>[4x]MSQHNEKNPHQHQSPLHDSSEAKPGMDSLAPEDGSHRPAAEPTPPGAQPTAPGSLKAPDTRNEKLNSLEDVRKGSENYALTTNQGVRIADDQNSLRAGSRGPTLLEDFILREKITHFDHERIPERIVNARGSAAHGYFQPYKSLSDITKADFLSDPNKITPVFVRFSTVQGGAGSADTVRDIRGFATKFYTEEGIFDLVGNNTPIFFIQDAHKFPDFVHAVKPEPHWAIPQGQSAHDTFWDYVSLQPETLHNVMWAMSDRGIPRSYRTMEGFGIHTFRLINAEGKATFVRFHWKPLAGKASLVWDEAQKLTGRDPDFHRRELWEAIEAGDFPEYELGFQLIPEEDEFKFDFDLLDPTKLIPEELVPVQRVGKMVLNRNPDNFFAENEQAAFHPGHIVPGLDFTNDPLLQGRLYSYTDTQISRLGGP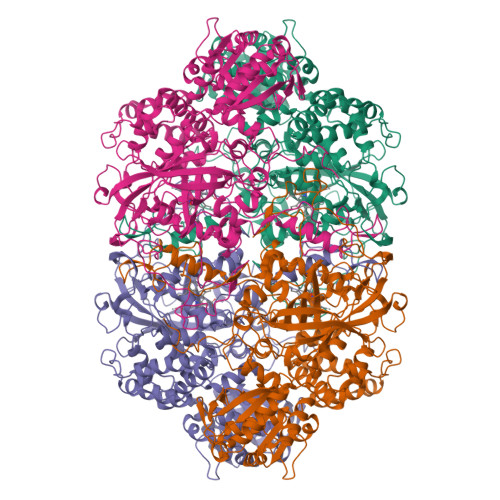NFHEIPINRPTCPYHNFQRDGMHRMGIDTNPANYEPNSINDNWPRETPPGPKRGGFESYQERVEGNKVRERSPSFGEYYSHPRLFWLSQTPFEQRHIVDGFSFELSKVVRPYIRERVVDQLAHIDLTLAQAVAKNLGIELTDDQLNITPPPDVNGLKKDPSLSLYAIPDGDVKGRVVAILLNDEVRSADLLAILKALKAKGVHAKLLYSRMGEVTADDGTVLPIAATFAGAPSLTVDAVIVPCGNIADIADNGDANYYLMEAYKHLKPIALAGDARKFKATIKIADQGEEGIVEADSADGSFMDELLTLMAAHRVWSRIPKIDKIPA>GSHMSSPRAEKARLYSAIEQRLEQSLQTMEGVLSARVHISYDIDAGENGRPPKPVHLSALAVYERGSPLAHQISDIKRFLK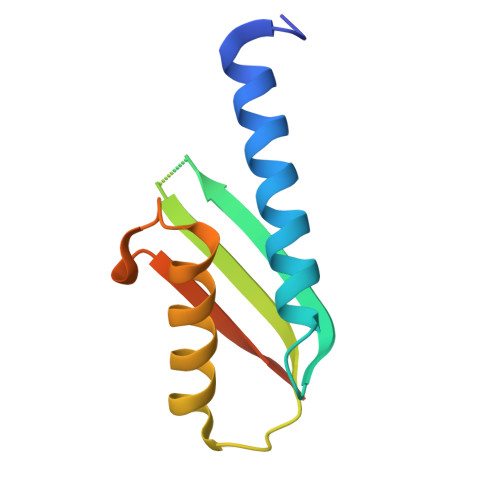NSFADVDYDNISVVLSERSDAQLQAPGT[2x]> MGSSHHHHHHSQDPVHFYETSYKYQAADSTYMHDVAINVSIKGNHFTSDIIIRELVKSENKNYYNVIGHGDIIQKNTHQYYLNFDNIDVYTGTNKANMKPYKEPTSISSLINKSNNIRVVYLSEE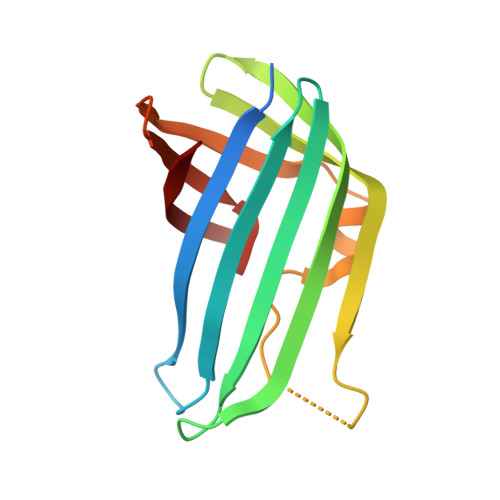YVVVEFFFYDGQIITLHRY>MKELIYIEEPSILFAHGQKCTDPRDGLALFGPLNQIYGIKSGVVGTQKGLQIFKSYLDKIQKPIYNHNNITRPMFPGFEAVFGCKWESQNIVFKEITDEEIRRYLFNASTHKRTYDLVTLFNDKIITANKNDEERVDVWFVIVPEEIYKYCRPNSVLPNELVQTKSLISKSKAKSFRYTPTLFEEFNKKLKEVEKEAKTYNYDAQFHDQLKARLLEHTIPTQILRESTLAWRDFKNTFGAPIRDFSKIEGHLAWTISTAAYYKAGGKPWKLGDIRPGVCYLGLVYKKIEKSKNPQNACCAAQMFLDNGDGTVFKGEVGPWYNPEKGEYHLKPKEAKALLTQALESYKEQNKSYPKEVFIHARTRFNDEEWNAFNEVTPKNTNLVGVTITKSKPLKLYKTEGAFPIMRGNAYIVDEKKAFLWTLGFVPKLQSTLSMEVPNPIFIEINKGEAEIQQVLKDILALTKLNYNACIYADGEPVTLRFANKIGEILTASTEIKTPPLAFKYYI[2x];>[2x]MRNKIFISHATPEDDDFTRWLSLKLIGLGYEVWCDILFLDKGVDFWSTIEKEIRENTCKFLIVSSTAGNKREGVLKELAVATKVKKHLQDDMFIIPLAIDENLSYDDINIEIVRLNAIDFKKSWAKGLQDLLDAFEKQNVPKKPPDHSKSNLLYQQIFLHDKQAIEKEETYDSNWFPIISFPNELRFHRYDWRLPKQFDVRTLAF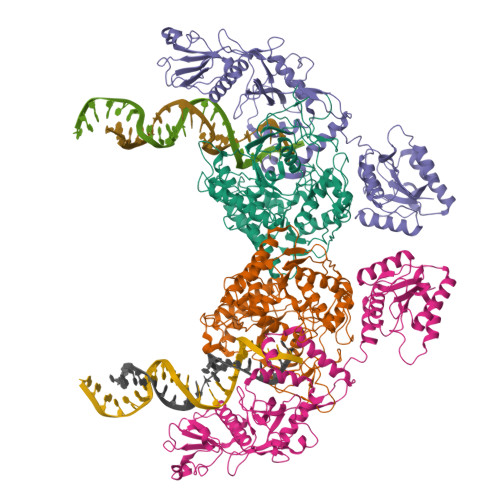PAIRYKEYLCTFAWEYDFIHQLPKTETYNGQESIRISTSDILSGRYDTDFIRNYECQRLIVQLINKAFELRMKDKNVREYQMSKTFAYWIEKGKLEKDKFEKIKLVGKQKNKYWHFGISAAGKLYPSPVLMVSSHIIFTMDGINLIKSKSIQHSSRRKQGKNWWNDKWREKLLAFIRFLSDDQNAIYLNVGSEEKILISNKPLKFFGKMSYVTPSEVTLEEESVLADINNFEEDTEDLDELEDIE> MAINVIINGINGKMGRVVKENITAQSDLELVSGTGRQDDLAKTIQTTHADVVIDFTTPQSVFHNAEIIIQSGARPVIGTTGLTLEQIALLDKQCRNKKLGAIV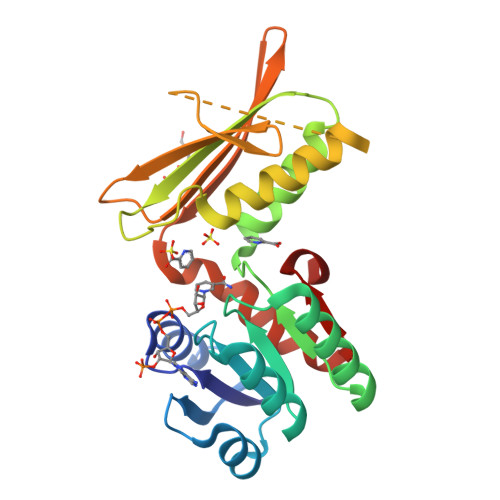APNFSVGAVLMMKYAKEAAHYFPDVEIIEMHHSQKIDAPSGTAIKTAQMIGEMRSSKKDEPFKDRARGEIKNGIPIHSIRLPGLFSHQSVIFGSNGETLTIRHDGMDRNCTMPGIFMACRKVMELDYLVYGLENLL> MGSTSTPDSSTNRLQDKVAIITGGAGGIGETTAKLFVRYGAKVVIADIADDHGQKVCNNIGSPDVISFVHCDVTKDEDVRNLVDTTIAKHGKLDIMFGNVGVLSTTPYSILEAGNEDFKRVMDINVYGAFLVAKHAARVMIPAKKGSIVFTASISSFTAGEGVSHVYTATKHAVLGLTTSLCTELGEYGIRVNCVSPYIVASPLLTDVFGVDSSRVEELAHQAANLKGTLLRAEDVADAVAYLA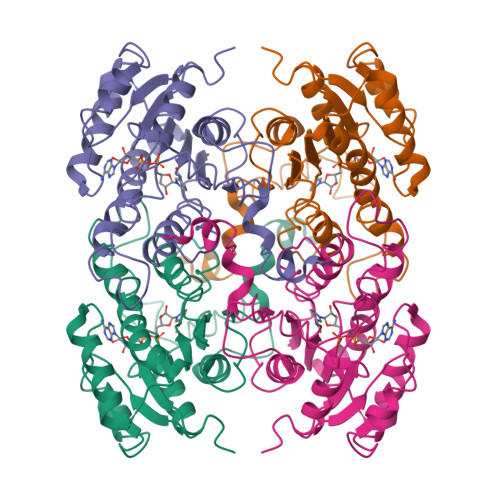GDESKYVSGLNLVIDGGYTRTNPAFPTALKHGLA> MKLRYLNILKEKLGREPTFVELQAFSVMWSEHCGYSHTKKYIRRLPKTGFEGNAGVVNLDDYYSVAFKIESANHPSAIEPYNGAATGVGGIIRDVLAMGARPTAIFDSLHMSRIIDGIIEGIADYGNSIGVPTVGGELRISSLYAHNPLVNVLAAGVVRNDMLVDSKASRPGQVIVIFGGATGRDGIHGASFASEDLTGDKATKLSIQVGDPFAEKMLIEAFLEMVEEGLVEGAQDLGAGGVLSATSELVAKGNLGAIVHLDRVPLREPDMEPWEILISESQERMAVVTSPQKASRILEIARKHLLFGDVVAEVIEEPVYRVMYRNDLVMEVPVQLLANAPEEDIVEYTPGKIPEFKRVEFEEVNAREVFEQYDHMVGTDTVVPP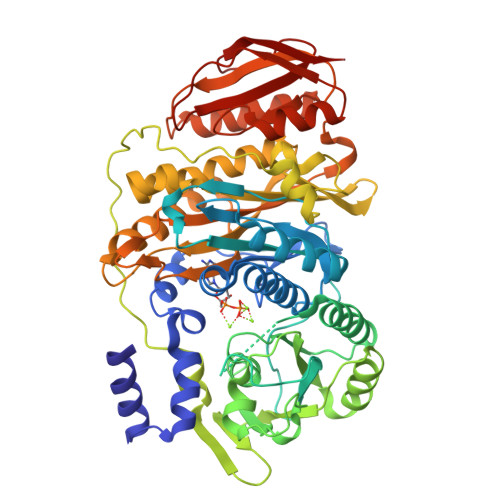GFGAAVMRIKRDGGYSLVTHSRADLALQDTYWGTLIAVLESVRKTLSVGAEPLAITNCVNYGDPDVDPVGLSAMMTALKNACEFSGVPVASGNASLYNTYQGKPIPPTLVVGMLGKVNPQKVAKPKPSKVFAVGWNDFELEREKELWRAIRKLSEEGAFILSSSQLLTRTHVETFREYGLKIEVKLPEVRPAHQMVLVFSERTPVVDVPVKEIGTLSR> SNESVD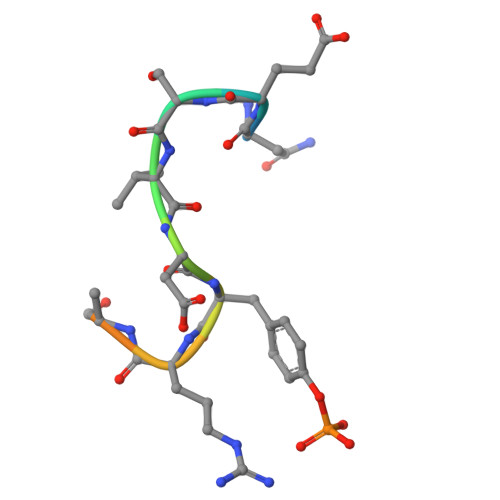YRATFPE>MSSASGLRRGHPAGGEENMTETDAFYKREMFDPAEKYKMDHRRRGIALIFNHERFFWHLTLPERRGTCADRDNLTRRFSDLGFEVKCFNDLKAEELLLKIHEVSTVSHADADCFVCVFLSHGEGNHIYAYDAKIEI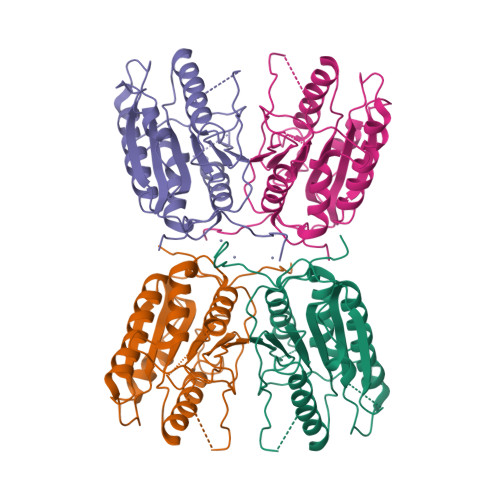QTLTGLFKGDKCHSLVGKPKIFIIQACRGNQHDVPVIPLDVVDNQTEKLDTNITEVDAASVYTLPAGADFLMCYSVAEGYYSHRETVNGSWYIQDLCEMLGKYGSSLEFTELLTLVNRKVSQRRVDFCKDPSAIGKKQVPCFASMLTKKLHFFPKSNHHHHHH[4x]> MLAKRIIAALIVKDGRVVKGSNFENLRDSGDP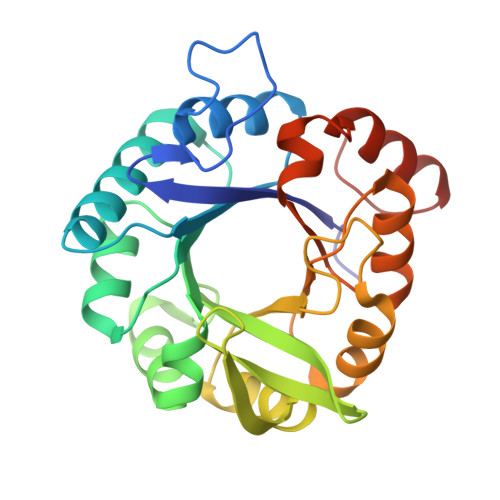VELGKFYSEIGIDELSFWDITASVEKRKTMLELVEKVAEQIDIPFTVGGGIHDFETASELILRGADKVEINTAAVENPSLITQIAQTFGSQAVVVYIAAKRVDGEFMVFTYSGKKNTGILLRDWVVEVEKRGAGEIVLGSIDRLGTKSGYDTEMIRFVRPLTTLPIIAHGGAGKMEHFLEAFLAGADAAKANSVFHFREIDVRELKEYLKKHGVNVRLEGLGS> 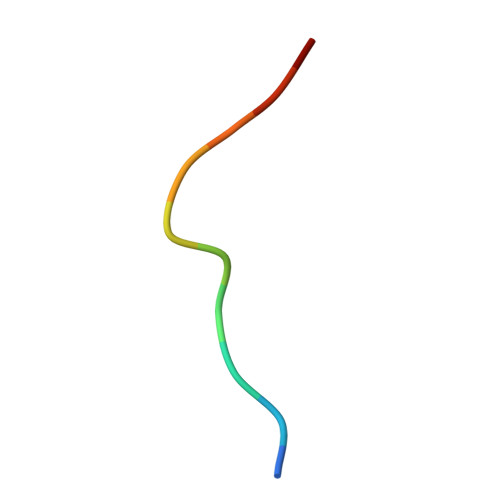GPRKCARKTRH> ETGHHHHHHSADEPMDFKINTDEIMTSLKSVNGQIESLISPDGSRKNPARNCRDLKFCHPELKSGEYWVDPNQGCKLDAIKVFCNMETGETCISANPLNVPRKHWWTDSSAEKKHVWFGESMDGGFQFSYGNPELPEDVLDVQLAFLRLLSSRASQQITYHCKNSIAYMDQASGNVKKALKLMGSNEGEFKAEGNSKFTYTVLEDGCTKHTGEWSKTVFEYRTRKAVRLPIVDIAPYDIGGPDQE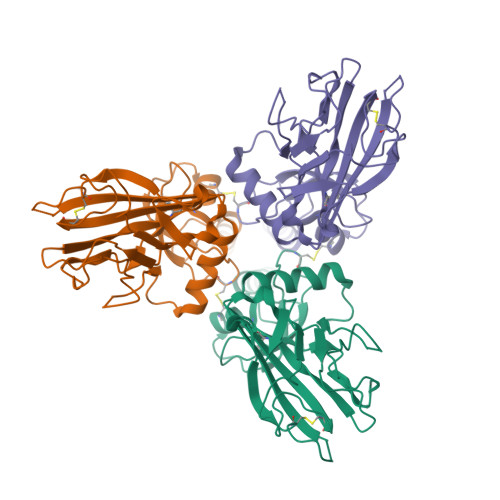FGVDVGPVCFL>[2x]MPLLDSFKVDHTKMNAPAVRIAKTMLTPKGDNITVFDLRFCIPNKEILSPKGIHTLEHLFAGFMRDHLNGDSIEIIDISPMGCRTGFYMSLIGTPNEQ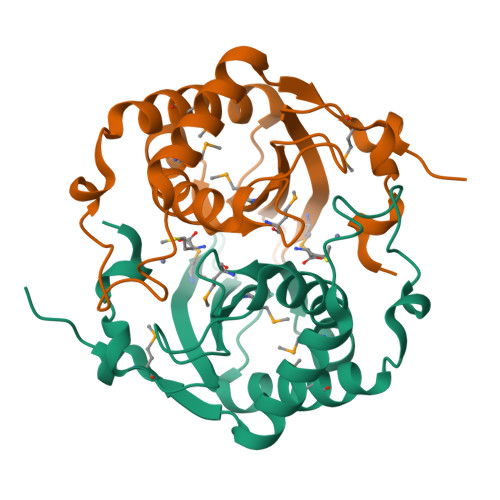KVSEAWLASMQDVLGVQDQASIPELNIYQCGSYTEHSLEDAHEIAKNVIARGIGVNKNEDLSLDNSLLKGSHHHHHH> MSPSVTEDAQWRHRRGLLPEGDPLVAALERLADRPRTHVFKAVGLIDAATGETAPPRDLEVADGVVAGWSPTPPVDGRPAPYDWYVTPGFVDAHAHVSSVSDLVGLLVHGVTAYRQLWGEPAHLLAAGVHRARHAVLPRPWVTAGVVDGPGSHVPQAATIVSGMRD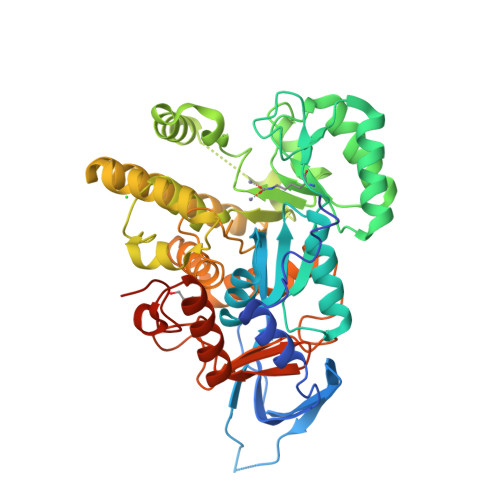VAKVVDDVLGFGFDGIKVYDDVERPVFEALVRDADRAGIPVVGHVPQAVRLDVALRTMRSTEHLYGFVPNVFRLPAAERWDALADALRHHHGDRLAEAAGHFVCPTLVAWRARTGERRFTRPSRAVLQAATPSRRPAWQAAARDALRLDPAEAERRGALVDRLGRIARALAEEGARLLVGTDCGNPFVVAGPSFHKEIAELTRAGLGFGAVLKAATADAYDVMGWHDKPAAGRADLVFYRRHPDDGPTGLARPDGVLVDGVFLDGEDLDRLWSLRLSAAGLDPSAWARGALDPPVTGARPDKEAAHAG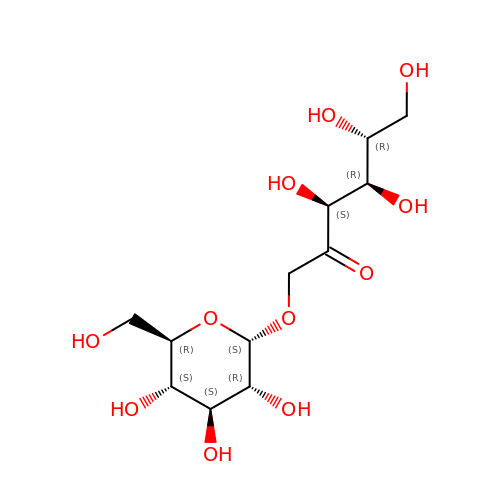1-O-alpha-D-glucopyranosyl-D-fructose | C12 H22 O11 | NMELTECMHKKXLF-DGQJZECASA-N>[2x]GSRIKQNPETTFEVYVEVAYPRTGGTLSDPEVQRQFPEDYSDQEVLQTLTKFCFPFYVDSLTVSQVGQNFTFVLTDIDSKQRFGFCRLSSGAKSCFCILSYLPWFEVFYKLLNILADYTTKRQENQWNELLETLHKLPIPDPGVSVHLSVHSYFTV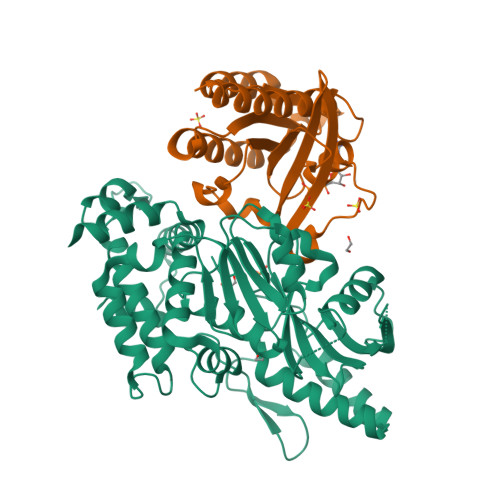PDTRELPSIPENRNLTEYFVAVDVNNMLHLYASMLYERRILIICSKLSTLTACIHGSAAMLYPMYWQHVYIPVLPPHLLDYCCAPMPYLIGIHLSLMEKVRNMALDDVVILNVDTNTLETPFDDLQSLPNDVISSLKNRLKKVSTTTGDGVARAFLKAQAAFFGSYRNALKIEPEEPITFCEEAFVSHYRSGAMRQFLQNATQLQLFKQFIDGRLDLLNSGEGFSDVFEEEINMGEY;>[2x]RDYDHLFKLLIIGDSGVGKSSLLLRFADNTFSGSYITTIGVDFKIRTVEINGEKVKLQIWDTAGQERFRTITSTYYRGTHGVIVVYDVTSAESFVNVKRWLHEINQNCDDVCRILVGNKNDDPERKVVETEDAYKFAGQMGIQLFETSAKENVNVEEMFNCITELVLRAKKDNLAK(3R)-3-hydroxybutyl 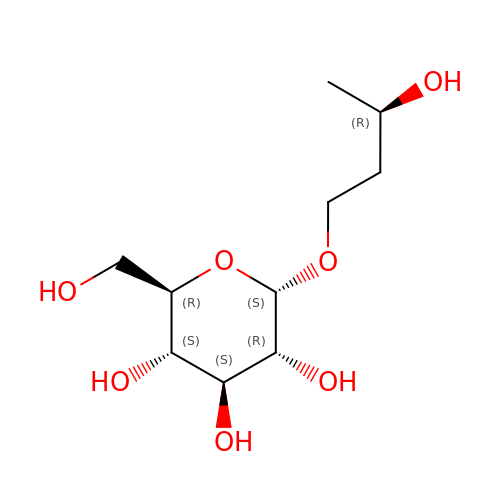alpha-D-glucopyranoside | C10 H20 O7 | IQTXPPTUXXJFDH-JQRWTQJCSA-N(2S)-2-[(4-CHLOROBENZYL)OXY]-2-PHENYLETHANAMINE | C15 H16 Cl 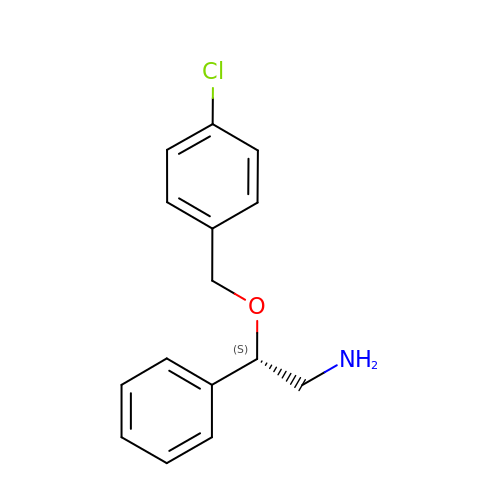N O | KFVPLCBTGAXYHI-OAHLLOKOSA-N4-hydroxy-3-methoxybenzaldehyde | C8 H8 O3 | 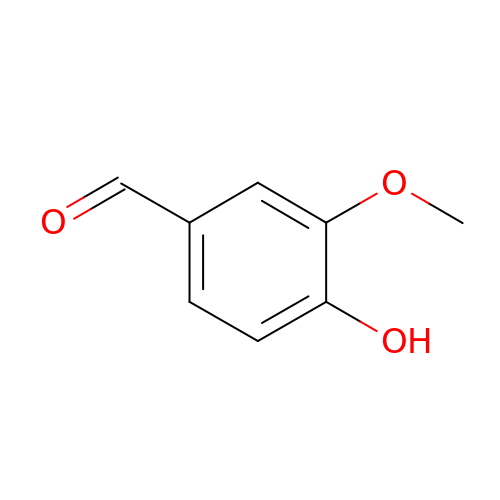MWOOGOJBHIARFG-UHFFFAOYSA-N>[2x]MNDSQTMLILLCNVNIYAPNPLGIKDVLIAGNKIAAIYDH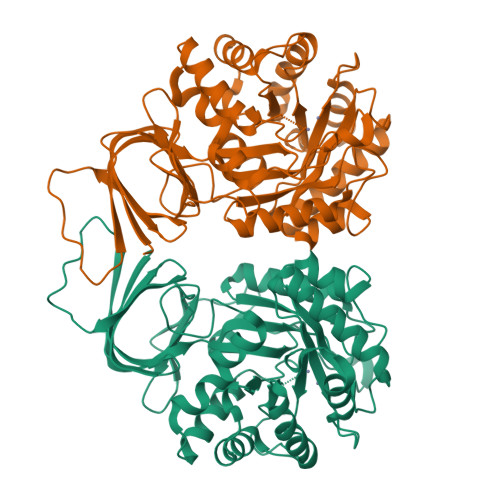GQGEITIPKQWPVKVINFDGAILTPGFIDSHAHITGGGGEAGFATQVPPVGLTEFTHAGVTTVVGLLGTDDTTRSTENLLSRVYGLREEGLSAYCWTGGYHFPLTTITGSAKSDIAFLEPVIGIGEFAISDHRSSQPTFEEVIRLASETHVAGLITGKAGVIHFHLGDGERRLELIERAIRETELPARVFNPTHVNRNKPLFEDSCKLLSKGCHIDLTAFPAGTAQPGWEACDAIEMAVERQLPLEQITLSSDGGGCLPCFDPQGELQHMDFGRASTLGETLVATLNKGLSLETVLPMLTSNVANILRFKNKGQIAVGFDADLLVMNEKYEITDVMAQGVWHKQNNQTMIKGTFE> MQDPIIKILIGNDTFLLGQEIIDLDFQIGEGKKQNNINFTIFDKDGFFADKYISTSYAQGGIDLPIDFLENPDDAKDTNSASTATEVDSVGNGTVSRSGVFTPKIRAFLDTIASKETAPGTALNIEGYRSVSGSSTLFDESEMVAGGFPRSQGSKNIGRYQFTVIDYNHARSKYPNINNYSPQNQDLLAYFKLQHRNVLPYLLRDDLDNAIDKASYEWASFPGIGKPQGQFNQVQSGTTIASLKSYYETRLAYYRSLEAGSDFQASAPKDTTNNQYAGKEYKTIRTLSNSTTASFYGYNDGFDSSDLTANGERFNPEGITAAHESLPFGTLVKVTWAVNNKS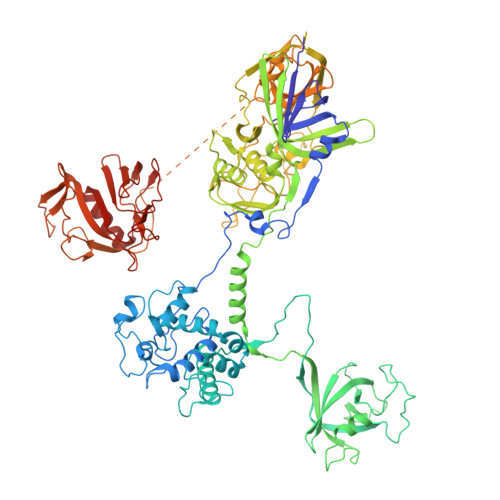VVVRINDRGAFVRLGRQIDLSYGAAKALSSPGNDAIAAGLLTVKLEVVELRTPIGENLKESAKNQIAENLEKIKKNQKELATPEISAKGTQITLEVSIDRSAIAVFSFLHTGTKHNAIISDTTTFTGQSVNWVLNRRVKNTRYTGVTLKGLAATITRQYGLDLDMSEEGEMIENISQVSQTDWQFLEKMTAIQGFGMRTVGKVLQIYKITVNAKKLNYTISVVDNVKSLIVTDQAQTDATGSSQKIEHYGGRMTTVVDADSGSLIKVDKDNKREAGSAARTFTTGVDVPQPQIQKQYSNPRPEGASVKEFQLQLELHTSQSDLENLTPDTALYIENTLPFIVGKSWFIESVRHSFSEGIFTSQVSAYIPVAPKAIATDSGEQNSVVFDNSQSASQGVGKLPVYEILSYRSGRTVKKITSLQQSYEHWRGTGGYTAYKQLSGFSSPVSYMKGRPNQLVYDFILQQNGNQSCPVPSPASGRVVATGGSNGMVKIDTGGGEVRLLHMSNIRVKPGQNVIRGTILGTQASVGGTSTGTHLHIEANQFILESYVQSLVTGNW> MEDAKNIKKGPAPFYPLEDGTAGEQLHKAMKRYALVPGTIAFTDAHIEVNITYAEYFEMSVRLAEAMKRYGLNTNHRIVVCSENSLQFFMPVLGALFIGVAVAPANDIYNERELLNSMNISQPTVVFVSKKGLQKILNVQKKLPIIQ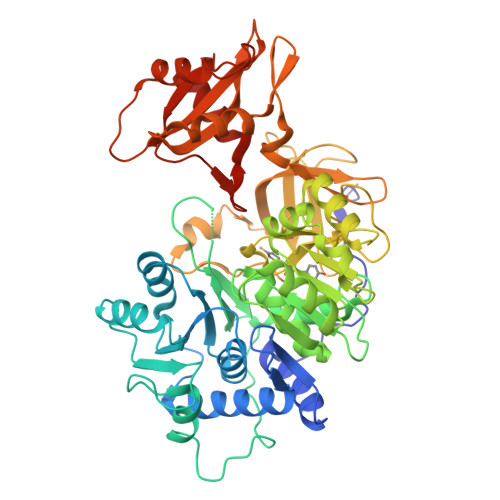KIIIMDSKTDYQGFQSMYTFVTSHLPPGFNEYDFVPESFDRDKTIALIMNSSGSTGLPKGVALPHRTACVRFSHARDPIFGNQIIPDTAILSVVPFHHGFGMFTTLGYLICGFRVVLMYRFEEELFLRSLQDYKIQSALLVPTLFSFFAKSTLIDKYDLSNLHEIASGGAPLSKEVGEAVAKRFHLPGIRQGYGLTETTSAILITPEGDDKPGAVGKVVPFFEAKVVDLDTGKTLGVNQRGELCVRGPMIMSGYVNNPEATNALIDKDGWLHSGDIAYWDEDEHFFIVDRLKSLIKYKGYQVAPAELESILLQHPNIFDAGVAGLPDDDAGELPAAVVVLEHGKTMTEKEIVDYVASQVTTAKKLRGGVVFVDEVPKGLTGKLDARKIREILIKAKKGGKSKL>GIDPFTGEDNGGEDNKKLRGALSSAILSEKPNVKWEDVAGLEGAKEALKEAVILPVKFPHLFKGNRKPTSGILLYGPPGTGKSYLAKAVATEANSTFFSVSSSDLVSKWMGESEKLVKQLFAMARENKPSIIFIDQVDALTGTRGEGESEASRRIKTELLVQMNGVGNDSQGVLVLGATNIPWQLDSAIRRRFERRIYIPLPDLAARTTMFEINVGDTPCVLTKEDYRTLGAMTEGYSGSDIAVVVKDALMQPIRKIQSATHFKDVSTEDDETRKLTPCSPGDDGAIEMSWT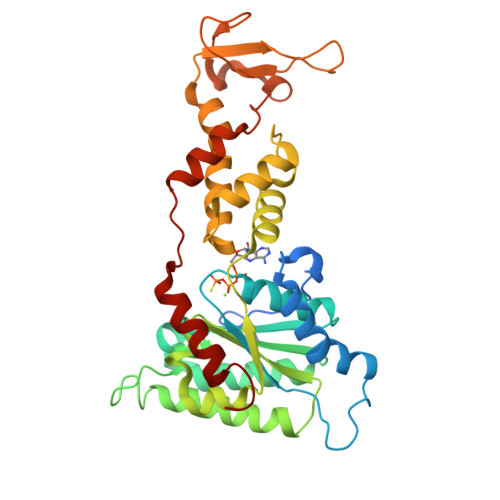DIEADELKEPDLTIKDFLKAIKSTRPTVNEDDLLKQEQFTRDFGQEGN[3x]> MRKTIIAGNWKMNLSLKEAVFLAHSIREKIPSISKDKVSMVFPSTLHLENVSKILEGSSVIVGAQNCYHSGLAAFTGETSPDQLKEIGVKVVMVGHSERRQFLGESNFFCNDKIRFLLKNEFTVLYC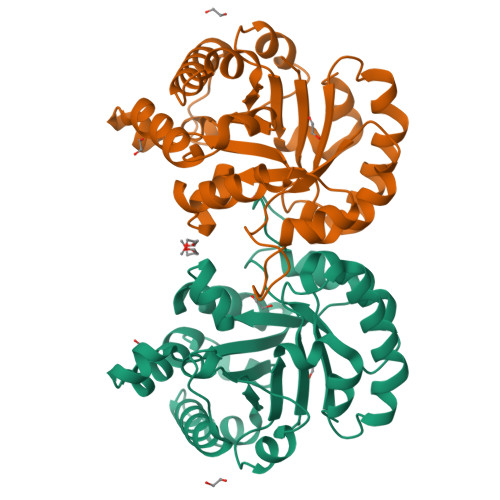VGETLSERESGKTLEVLSSQIREGLKGIDSVFFSNLILAYEPVWAIGTGKVATPSQAQEVHSFIRKEISGLFVGASSISESISILYGGSVKPDNIQDLLKEKDIDGGLVGGASQKISSFAGLF> VCNRLEQILVKTQWAQSYGEAENRAAFSRDLFSELFNIQGSSRALFSGVGVDDMNSAAFTAHCLRVTGALNRLISQLDQQATINADLAHLAGQHASRNLDASNFAAMGQAVMSVVPTHLDCFNQHAWGECYERIASGISG;> DCTSLNRLLVKRQWAEAYGEGTNRELLGNRIWEDLFANMPDARGLFSRVNGNDIDSSEFQAHSLRVLGGLDMCVASLDDVPVLNALLARLNSQHDSRGIPAAGYPAFVASAISAVRATVGARSFDNDAWNSCMNQIVSGISG;> SSCCSSEDRANVMHNWDAAWSAAYSDRRVALAQAVFASLFSRDAAAQGLFSGVS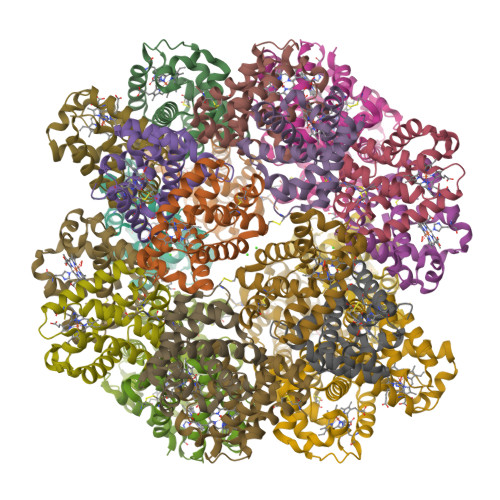ADNPDSADFRAHCVRVVNGLDVAINMLNDPAVLNEQLAHLSAQHQARAGVAAAHFDVMAEAFAEVMPQVSSCFSSDSWNRCFARIANGISAGL;> ECCSRGDAEVVISEWDQVFNAAMAGSSESAIGVAIFDVFFTSSGVSPSMFPGGGDSSSAEFLAQVSRVISGADIAINSLTNRATCDSLLSHLNAQHKAISGVTGAAVTHLSEAISSVVAQVLPSAHIDAWGYCMAYIAAGIGAGL> MTNNKYTNRPIHQLQELLRLNGVDEEWEPILLPALMTLEDSYLEWMAAGEGYI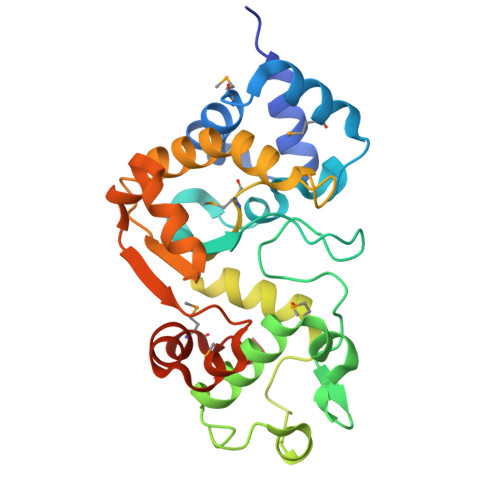PPRDRLLAAFSTLRPNEVRYILFGQDPYPRPESAIGYAFIDGRVREIFSPRGLSREVNRATSLRNFIKMALVARGSLDPRDTSQEAIAALDKTLLVSQMRELRENFERSGVLLLNMALLFTSKEESRRHIRAWRAFIEKLLEGFEAYGPTLILFGAHAREVQKLKSARGLPQVALEHPYNHTFIVNEKAWELFGPMDLLLKRLEHHHHHH> MDTSLIRELAELALAGSGQ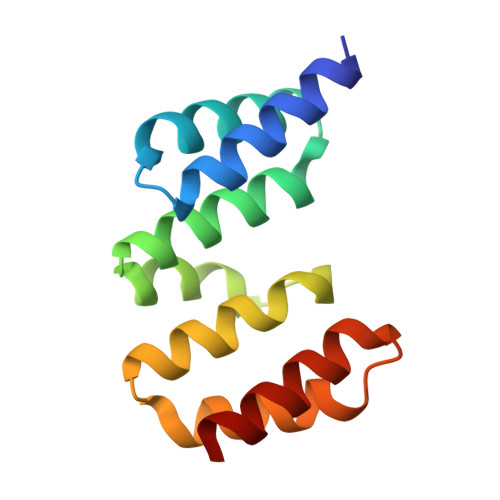HCHEEALCIAEWLERLGQDEAARLIRISSLANQGRYQEALAFAHGNPWPALEPWFALCEWHLGLGAALDRRLAGLGGSSDPALADFAAGMRAQVRT>[2x]HMKIAVMTDSTSYLSQDLIDKYNIQIAPLSVTFDDGKNFTESNEIAIEEFYNKMASSQTIPTTSQPAIGEWITKYEMLRDQGYTDIIVICLSSGISGSYQSSYQAGEMVEGVNVHAFDSKLIAMIEGCYVLRAIEMVEEGYEPQQIIDDLTNMREHTGAYLIVDDLKN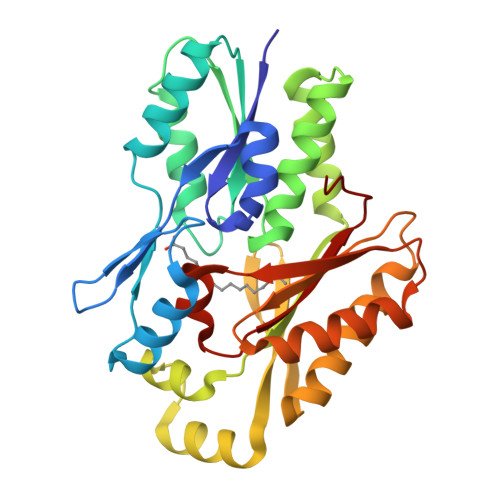LQKSGRITGAQAWVGTLLKMKPVLKFEDGKIIPEEKVRTKKRAIQTLEKKVLDIVKDFEEVTLFVINGDHFEDGQALYKKLQDDCPSAYQVAYSEFGPVVAAHLGSGGLGLGYVGRKIRLT>[2x]PCPAPCSCAGTLVDCGRRGLTWASLPTAFPVDTTELVLTGNNLTALPP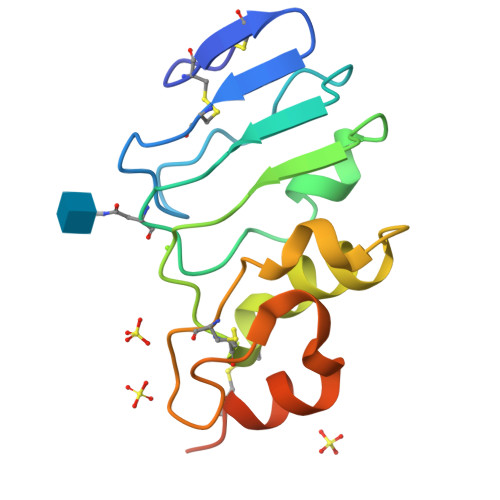GLLDALPALRTAHLGANPWRCDCRLVPLRAWLAGRPERAPYRDLRCVAPPALRGRLLPYLAEDELRAACAPGPLSSHHHHHH> CTKSIPP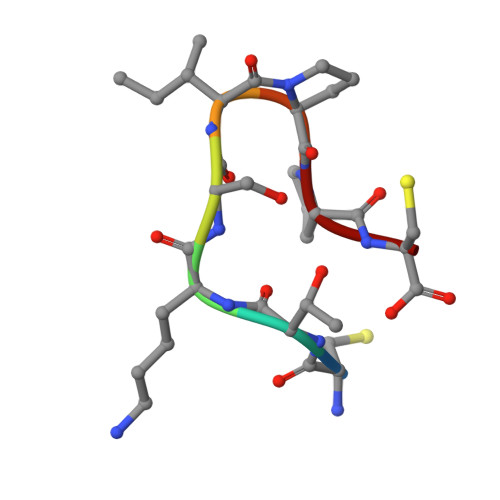C>[2x]MLSLTRILRKKIPVHELAGKISRPPLRPFSVVVASDEKGGIGDGGTIPWEIPEDMQYFRRVTTNLRGKN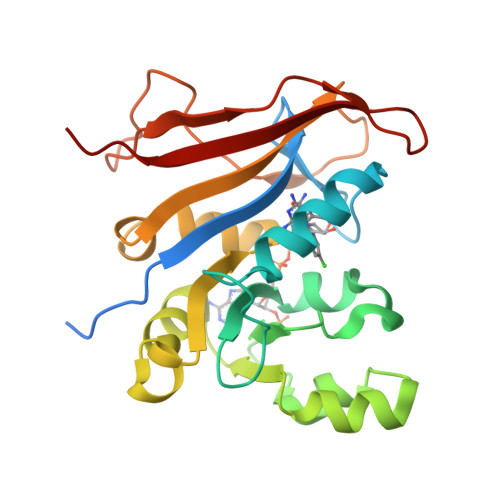VKPSPSKRNAVVMGRKTWDSLPPKFRPLSNRLNVVLSRSATKEQLLAGIPDPIKRAEAANDVVAVNGGLEDALRMLVSKEHTSSIETVFCIGGGTIYKQALCAPCVNVLQAIHRTVVRPASNSCSVFFDIPAAGTKTPEGLELVRESITDERVSTGAGGKKYQFEKLVPRNS Here, we report, at a resolution of 1.5 Å, the crystal structure of DynU16, a putative di-domain protein homolo­gous to StAR-related lipid-transfer (START/Bet v1-like) domain-containing proteins. The enediyne core is synthesized by a type I highly reducing iterative polyketide synthase (iPKS), yielding a linear conjugated polyene upon release from the iPKS by a thioesterase. While an actual enzymatic assay is needed to confirm the speculated function of DynU16, we conclude that it is likely that this protein participates in the biosynthesis of dynemicin as a cyclase or perhaps at least as a dehydratase of an extended or cyclic ANQ precursor.

The final model included 269 protein residues, 282 water molecules and five ions. Residues 0 (left from the tag after cleavage) to 8 at the N-terminus and 278–283 at the C-terminus were disordered and were not modeled. The N-terminal (residues 1–139) and C-terminal (residues 150–283) domains are connected by a flexible ten-residue linker (140–149). Assessment of the C-terminal domain suggests divergence from the canonical START/Bet v1 fold observed in the N-terminal domain. The C-terminal domain possesses eight instead of six antiparallel β-strands and has adopted additional loops. The opposing region of the cavity is composed of aromatic residues, including Phe57, Phe63, Phe82, Phe128, Trp80, Trp125 and Tyr144. The abundance of aromatic residues localized in one region of the cavity suggests a possible role in carbocation intermediate stabilization if cyclization is catalyzed in the cavity. The cavity-forming residues frequently reside in loops or β-strands, potentially increasing cavity flexibility and enabling contraction and expansion to accommodate substantial substrate rearrangements. The shape and size of the cavity appears to support the binding of a linear or perhaps a cyclic polyene.

> SMPDGYLKLPDDWVRVMVSVPAPVDEVWEAVTDPRRVAQWFGHLSAPMTTGASTRVDFGDGDFFDIEVDHVEPRDRLLFRWSFLGVGPECQVGWTLTGGAEATTLTVDDSCPGRPGSEVAQLKAGWLDFVGRLARYLETGKPSRYDWRQEIDGSVVLPNGSWHPLREETVVDWLPIATNGAGPGWFFVVDEEGPRRFTLRDWQLDRERALTFAVEIPGARTVTACQVRTEPGERGRTLSVSHQGWHRLGLSDLQERTLRHRFAATWTAALSLAEECARTRQELP>MRGSHHHHHHYVAALFFLIPLVALGFAAANFAAVVRKPEGTERMKEISSYIRSGADSFLAHETKAIFKVAIVIAILLMIFTTWQTGVAFLLGAVMSASAGIVGMKMATRANVRVAEAARTTKKIGPALKVAYQGGSVMGLSVGGFALLGLVLVYLIFGKWMGQVDNLNIYTNWLGINFVPFAMTVSGYALGCSIIAMFDRVGGGVYTKAADMAADLVGKTELNLPEDDPRNPATIADNVGDNVGDVAGLGADLLESFVGAIVSSIILASYMFPIYVQKIGENLVHQVPKETIQALISYPIFFALVGLGCSMLGILYVIVKKPSDNPQRELNISL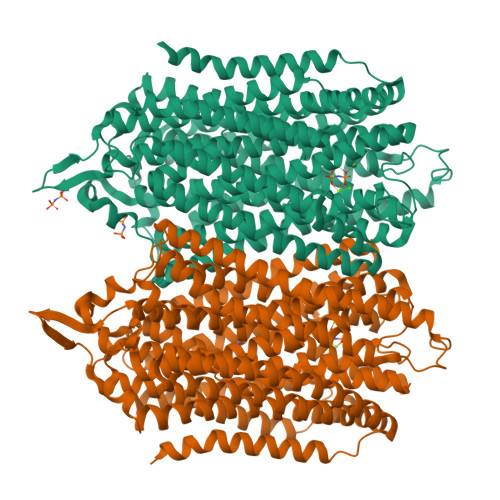WTSALLTVVLTAFLTYFYLKDLQGLDVLGFRFGAISPWFSAIIGIFSGILIGFWAEYYTSYRYKPTQFLGKSSIEGTGMVISNGLSLGMKSVFPPTLTLVLGILFADYFAGLYGVAIAALGMLSFVATSVSVDSYGPIADNAGGISEMCELDPEVRKITDHLDAVGNTTAAIGKGFAIGSAIFAALSLFASYMFSQISPSDIGKPPSLVLLLNMLDARVIAGALLGAAITYYFSGYLISAVTKAAMKMVDEIRRQAREIPGLLEGKAKPDYNRCIEITSDNALKQMGYPAFIAILTPLVTGFLLGAEFVGGVLIGTVLSGAMLAILTANSGGAWDNAKKYLEAGNLEGYGKGSEPHKALVIGDTVGDPLKDTVGPSLDILIKIMSVVSVIAVSIFKHVHLF[2x]>MKQVKIMFLMTMFLGIGLLFFSENAEAAITSNEIGTHDGYDYEFWKDSGGSGSMTLNSGGTFSAQWSNVNNILFRKGKKFDETQTHQQIGNMSINYGATYNPNGNSYLTVYGWTVDPLVEFYIVDSWGTWRPPGGTPKGTINVDGGTYQIYETTRYNQPSIKGTATFQQYWSVRTSKRTSGTISVSEHFRAWESLGMNMGNMYEVALTVEGYQSSGSANVYSNTLTIGGQSGGEQATRVEAESMTKGGPYTSNITSPFNGVALYANGDNVSFNH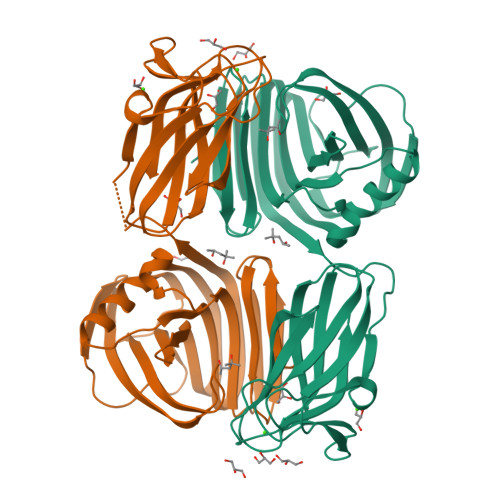SFTKANSSFSLRGASNNSNMARVDLRIGGQNRGTFYFGDQYPAVYTINNINHGIGNQLVELIVTADDGTWDAYLDYLEIR[2x]> MADEALFLLLHNEMVSGVYKSAEQGEVENGRCITKLENMGFRVGQGLIERFTKDTARFKDELDIMKFICKDFWTTVFKKQIDNLRTNHQGIYVLQDNKFRLLTQMSAGKQYLEHASKYLAFTCGLIRGGLSNLGIK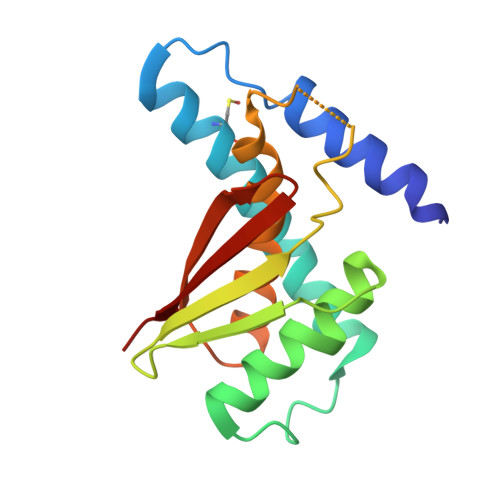SIVTAEVSSMPACKFQVMIQKL>[2x]GAMATPWRNPAEEREKLAYRKQNMDDIDEEDDDLVGVSVRPKVPLRTM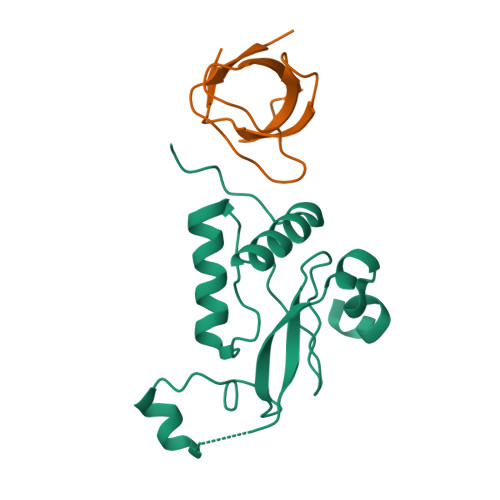SYKLAIDMSHFIKEKGGLEGIYYSARRHRILDIYLEKEEGIIPDWQDYTSGPGIRYPKTFGWLWKLVPVNVSDEAQEDEEHYLMHPAQTSQWDDPWGEVLAWKFDPTLAYTYEAYVRYPEEFGS;>[2x]MEDIIVVALYDYEGWWGDLSFQKGDQMVVLEESGEWWKARSLATRKEGYIPSNYVARVDS> NETEA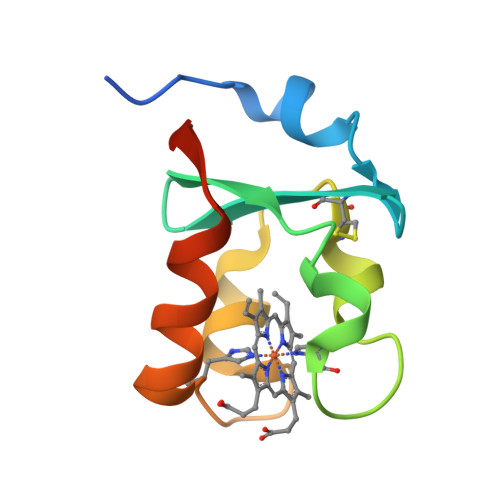TLPVFTLEQVAEHHSPDDCWMAIHGKVYDLTPYVPNHPGPAGMMLVWCGQESTEAWETKSYGEPHSSLAARLLQRYLIGTLEEIT> XMLKLRQLQKKK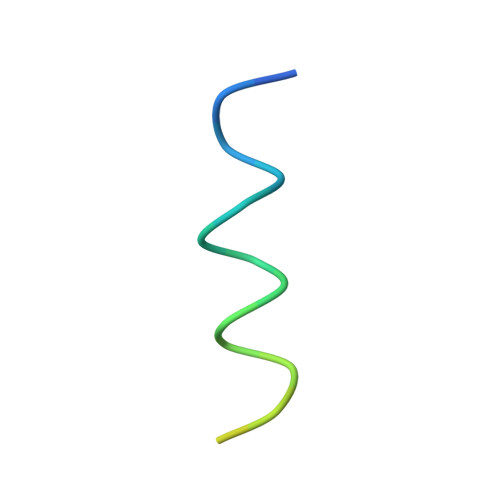QKENENSSSIQPN> MGSSHHHHHHSQDPMVLLHKSTHIFPTDFASVSRAFFNRYPNPYSPHVLSIDTISRNVDQEGNLRTTRLLKKSGKLPTWVKPFLRGITETWIIEVSVVNPAN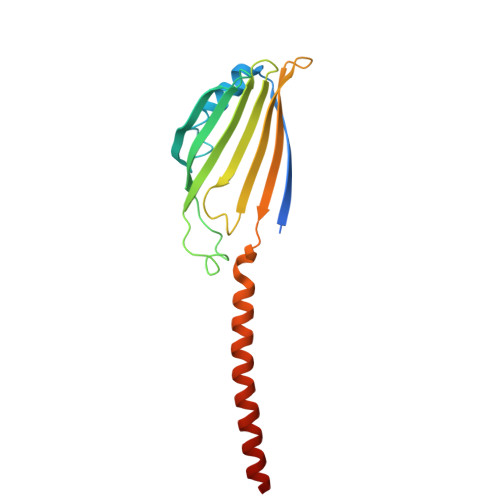STMKTYTRNLDHTGIMKVEEYTTYQFDSATSSTIADSRVKFSSGFNMGIKSKVEDWSRTKFDENVKKSRMGMAFVIQKLEEA> 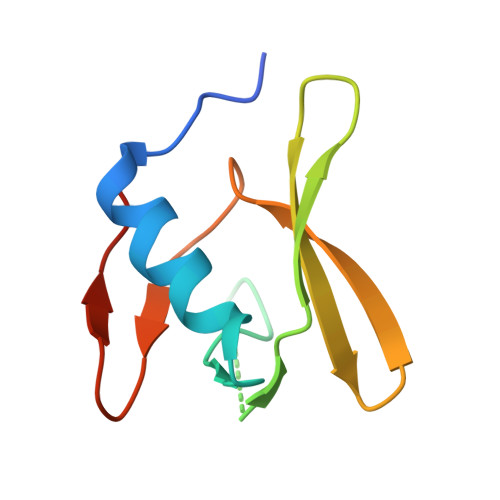MNDTYQPINCDDYDNLELACQHHLMLTLELKDGEKLQAKASDLVSRKNVEYLVVEAAGETRELRLDKITSFSHPEIGTVVVSES> QDLTVKMTDLQTGKPVGTIELSQNKYGVGFIPELADLTPGMHGFHIHQNGSCASSEKDGKVVLGGAAGGHYDPEHTNKHGFPWTDDNHKGDLPALFVSANGLATNPVLAPRLTLKELKGHAIMIHAGGDNH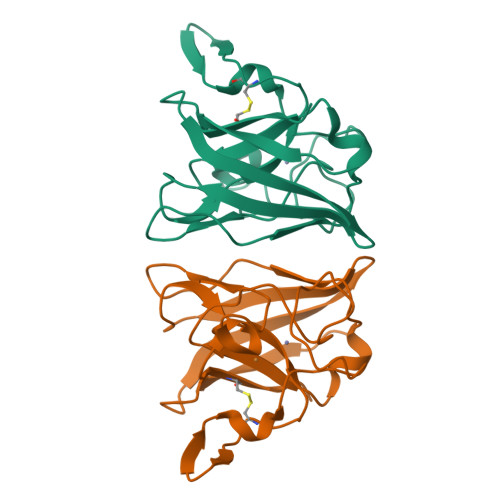SDMPKALGGGGARVACGVIQ>MGIPILKLGECLLISIQSELDDHTAVEFQEDLLAKIHETSARGVVIDITSIDFIDSFIAKILGDVVSMSKLMGAKVVVTGIQPAVAITLIELGITFSGVLSAMDLESGLEKLKQELGE[20x];>[30x]SALQELSAPLLPIFEKISVMPLIGTIDTERAKLIIENLLIGVVKNRSEVVLIDITGVPVVDTMVAHHIIQASEAVRLVGCQAMLVGIRPEIAQTIVNLGIELDQIITTNTMKKGMERALALTNREIVE;> EKTVSIQKSALQELSAPLLPIFEKISVMPLIGTIDTERAKLIIENLLIGVVKNRSEVVLIDITGVPVVDTMVAHHIIQASEAVRLVGCQAMLVGIRPEQIITTNTMKKGMERALALTNREIVE;>[6x]KSALQELSAPLLPIFEKISVMPLIGTIDTERAKLIIENLLIGVVKNRSEVVLIDITGVPVVDTMVAHHIIQASEAVRLVGCQAMLVGIRPEIAQTIVNLGIELDQIITTNTMKKGMERALALTNREIVE;>[3x]EKTVSIQKSALQELSAPLLPIFEKISVMPLIGTIDTERAKLIIENLLIGVVKNRSEVVLIDITGVPVVDTMVAHHIIQASEAVRLVGCQAMLVGIRPEIAQTIVNLGIELDQIITTNTMKKGMERALALTNREIVE

In bacteria, the stressosome, a key inducer of the stress response is a very large nanomachine that responds to diverse environmental changes by triggering a protein partner-switching cascade of events, which culminate in the desequestration and activation of an alternative sigma factor. Here, in a first step toward understanding the molecular details of stressosome activation, we report an atomic resolution cryo-EM structure of the L. monocytogenes stressosome. The stressosome contains 20 dimers of RsbR and 10 dimers of RsbS, arranged in repeating units of 2 dimers of RsbR and 1 dimer of RsbS. The L. monocytogenes stressosome core proteins, RsbR and RsbS, display the signature β-strands-α-helical arrangement of a typical STAS domain where a central 4-stranded β-sheet is flanked by one α-helix on one side and three α-helices on the other.

Next, to improve the resolution in the core structure, icosahedral symmetry (demonstrated by Marles-Wright et al. in their study of the B. subtilis stressosome core) was applied during the 3D refinement using a mask that excluded the turrets, yielding a 3.38 Å resolution map. In the latter map, the density for the C-terminal domain of RsbR is well defined, even for side chains, allowing the structure of this RsbR domain to be built. The STAS domains of RsbR and RsbS each form head to head homodimers. The total buried surface area of the interface between the RsbR STAS domains within the RsbR dimer is 1027.3 Α2 while that within the RsbS dimer is 657.6 Α2. This difference in surface area buried upon dimerization is partly due to the fact that the C-terminal tails of the STAS domains in each RsbR subunit overlap to form a large interlocking interface, absent in RsbS. All dimer–dimer interfaces, whether between RsbR dimers or between RsbR and RsbS dimers, involve residues in helical secondary structures and flexible loops (helix α2 and the flexible loop region between helices α3 and α4, for example). This is in contrast with the fact that interfaces within RsbR and RsbS homodimers are formed by residues in β-strands. In our model, the phosphorylation sites of RsbR and RsbS are clustered at the dimer–dimer interface of RsbR and RsbS. Interestingly, T209 of RsbR a key residue in stressosome activation is located near the flexible loop between helices α3 and α4 (the α3–α4 loop) of RsbR between residue 237 and 251 region that is disordered. Therefore, this loop could adopt two conformations, one (closed) preventing RsbT access to T209 and one (open) allowing access.> MEVSNDIPNDEAGNQPIELATRSVGGSGSVGGGGRGGSGVGYSTGGWTGGTIFSENIVVTKNTRQFICDIKNGHLYKSEVLNTGDTAHRQYAITTPWSYFNFNQYSSHFSPNDWQHLVNDYERFRPKAMIVRVYNLQIKQIMTDGAMGTVYNNDLTAGMHIFCDGDHRYPYVQH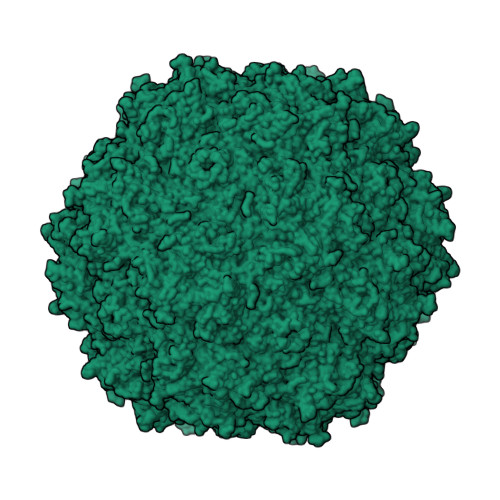PWDDQCMPELPNSIWELPQYAYIPAPISVVDNNTTNTVEEHLLKGVPLYMLENSDHEVLRTGESTEFTFNFGDCEWIENNITFSMPQMMYNPLVRSRRIYSYSGPNNQTSNAFQNAALRTSNWMSGPGIARGTHNATLQTQSAGALVTMVTNGADVSGVGAVRVGYSTDPIYGGQQPDSDLLRLRYSASAAEGQQNPILENAARHTFTREARTKLITGSNGADGNYKEWWMLPNQMWDSAPISRYNPIWVKVPRVNRKTLLDTQDGSIPMSHPPGTIFIKLARIPVPGNGDSFLNIYVTGQVSCEVVWEVEKRGTKNWRPEYMHSATNMSVDAYTINNAGVYAGAVQNADVMQTRFNHHKVL>MTNGDNLAQIGVVGLAVMGSNLARNFARNGNTVAVYNRSTDKTDKLIADHGSEGNFIPSATVEEFVASLEKPRRAIIMVQAGNATDAVINQLADAMDEGDIIIDGGNALYTDTIRREKEISARGLHFVGAGISGGEEGALNGPSIMPGGPAKSYESLGPLLESIAANVDGTPCVTHIGPDGAGHFVKMVHNGIEYADMQVIGEAYHLLRYAAGMQPAEIAEVFKEWNAGDLDSYLIEITAEVLSQVDAETGKPLIDVIVDAAGQKGTGRWTVKAALDLGIATTGIGEAVFARALSGATSQRAAAQGNLPAGVLTDLEALGVDKAQFVEDVRRALYASKLVAYAQGFDEIKAGSDENNWDVDPRDLATIWRGGCIIRAKFLNRIVEAYDANAELESLLLDPYFKSELGDLIDSWRRVIVTATQLGLPIPVFASSLSYYDSLRAERLPAALIQGQRDFFGAHTYKRIDKDGSFHTEWSGDRSEVEALEHHHHHH[2x]

In summary, we determined the crystal structures of the apo and complex forms of Cg6PGD with a resolution of 2.4 and 1.9 Å, respectively; Cg6PGD is the crucial enzyme in NADPH production. Cg6PGD eluted with a molecular weight of approximately 116.8 kDa, indicating that Cg6PGD exists as a dimer in solution. The monomeric structure of Cg6PGD could be divided into three functional domains : the N-terminal domain (N-term domain, Met1-Pro179), the central domain (CD, Asp180-Arg441), and the C-terminal domain (C-term domain, Ala442-Ala484). The CD consisted of α-helices exclusively and was associated with dimerization.

Structural differences between Cg6PGD_apo and Cg6PGD_NADP were detected in the residual movement together with the loop. A NADP-binding site was observed in the N-term domain. The N-term domain consists of seven β-strands surrounded by seven α-helices and was associated with NADP-binding. The NADP-binding site was constructed by Ala16, Met18, Asn37, Arg38, Ser39, Lys42, Val79, Gln80, Asn107 and Glu136. Among these residues, Arg38, Ser39 and Lys42 were crucial for binding to NADP. The guanidinium group of Arg38 established a stable π -cation interaction with the adenine ring of NADP, and the π-cation interaction and hydrogen bonds that formed between Arg38 and NADP played an important role in the stable cofactor binding of Cg6PGD. Asn107 interacts with 6PG and cooperates with Met18 to form a shallow cavity for NADP-binding. A structural comparison between the docking simulation of 6PG and Cg6PGD_NADP showed that the nicotinamide ring of NADP and the carboxylate group of 6PG are positioned in parallel, to achieve electron transfer. By checking our Cg6PGD_NADP-binding form, we found that Cg6PGD had class I that is typical of NAD(P)-binding proteins. The analysis of the structure of Cg6PGD_NADP made it appearent that Thr and His prevented the binding of NADP.> GSHMPPNRPGITFEIGARLEALDYLQKWYPSRIEKIDYEEGKMLVHFER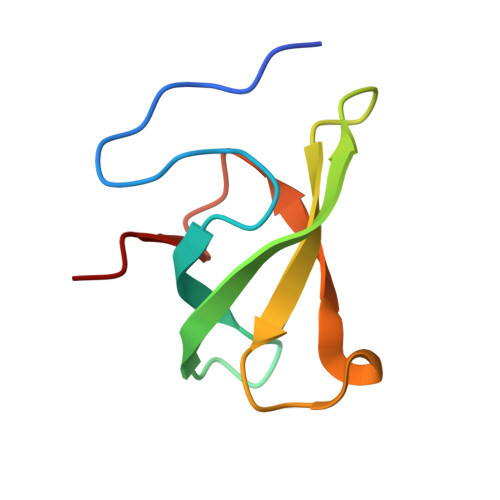WSHRYDEWIYWDSNRLRPLER Contrasting with Enterobacteria, members of the dominant genus Bacteroides often encode several BtuB vitamin B12 outer membrane transporters together with a conserved array of surface-exposed B12-binding lipoproteins. Here we show that the BtuB transporters from Bacteroides thetaiotaomicron form stable, pedal bin-like complexes with surface-exposed BtuG lipoprotein lids, which bind B12 with high affinities. Closing of the BtuG lid following B12 capture causes destabilisation of the bound B12 by a conserved BtuB extracellular loop, causing translocation of the vitamin to BtuB and subsequent transport. We propose that TonB-dependent, lipoprotein-assisted small molecule uptake is a general feature of Bacteroides spp. that is important for the success of this genus in colonising the human gut.

As observed previously, CNCbl binds to BtuG2 with very high affinity. The BtuG2-CNCbl complex is extremely stable, given that a boiled sample run on a denaturing SDS-PAGE gel shows a visible pink band around 40 kDa, suggesting that some CNCbl is still bound to BtuG2. An initial BtuG2-CNCbl structure was solved to 1.9 Å resolution using cobalt-based single-wavelength anomalous diffraction (Co-SAD), showing unambiguous electron density for CNCbl. This model was used to solve an additional dataset at slightly higher resolution (1.7 Å). BtuG2 adopts a seven-bladed beta-propeller fold. The propeller blades define a central cavity that forms the B12 binding pocket with an interface area of 698 Å2 as measured via PISA22. CNCbl is oriented with the cyano group (upper ligand) pointing towards the protein centre while the lower ligand, present in its “base-on” conformation, is completely exposed to the exterior, with the nucleotide loop sitting in the cleft formed between blades 1 and 7. There are 13 hydrogen bonds between BtuG2 and CNCbl, all mediated by the amide groups of the substituents from side chains a, b, c and g of the corrin ring and involving protein residues from blades 1 to 4. CNCbl binding is further stabilised by Van der Waals forces provided by 11 residues, evenly distributed across the blades. The cavity that contains the cyano upper ligand is narrowed by Trp194, Trp272 and Tyr316 (numbering based on the annotated Uniprot sequence, including the signal peptide).

>[2x]CMKWDYGEMEDFSVSASGLFITNEGNFQYSNATLSYYDPATCEVENEVFYRANGFKLGDVAQSMVIRDGIGWIVVNNSHVIFAIDINTFKEVGRITGFTSPRYIHFLSDEKAYVTQIWDYRIFIINPKTYEITGYIECPDMDMESGSTEQMVQYGKYVYVNCWSYQNRILKIDTETDKVVDELTIGIQPTSLVMDKYNKMWTITDGGYEGSPYGYEAPSLYRIDAETFTVEKQFKFKLGDWPSEVQLNGTRDTLYWINNDIWRMPVEADRVPVRPFLEFRDTKYYGLTVNPNNGEVYVADAIDYQQQGIVYRYSPQGKLIDEFYVGIIPGAFCWKLEHHHHHH>HMMASVELSADVPISPQDTWDHVSELSELGEWLVIHEGWRSELPDQLGAGVQIVGVARAMGMRNRVTWRVTKWDPPHEVAMTGSGKGGTKYGVTLTVRPTKGGSALGLRLELGGRALFGPLGSAAARAVKGDVEKS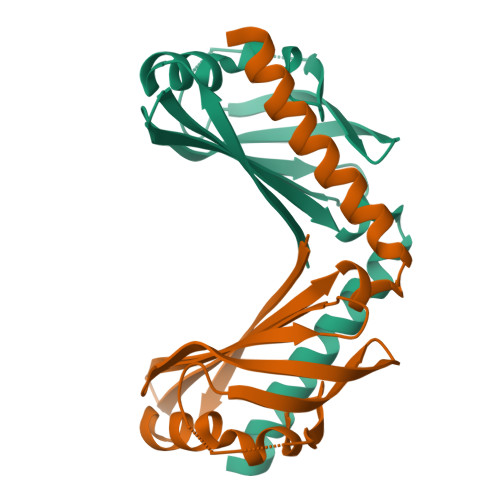LKQFAELY[2x]4-[(E)-(3,5-DIAMINO-1H-PYRAZOL-4-YL)DIAZENYL]PHENOL | C9 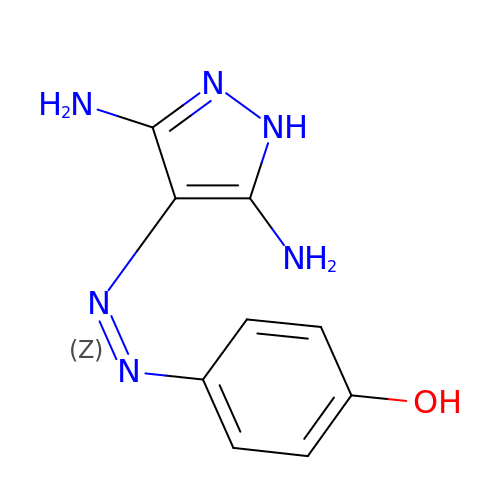H10 N6 O | AYZRKFOEZQBUEA-SEYXRHQNSA-N>[2x]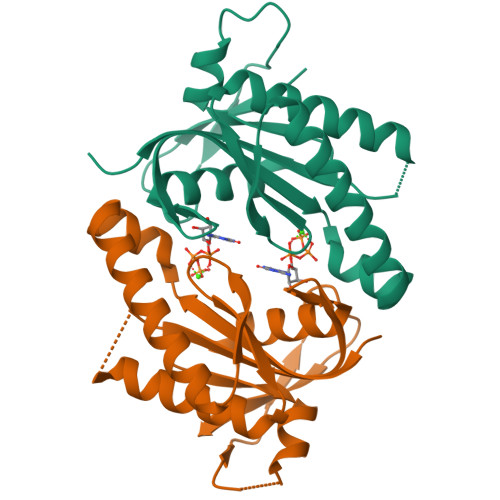FQGAMGSRVVILFTDIEESTALNERIGDRAWVKLISSHDKLVSDLVRRQSGHVVESQGDGFMVAFARPEQAVRCGIELQRALRRNANRKRHEEIRVRIGIHMGRSVRRGDGLFGRNVAMAYRVAAQAAGGEILVSQPVRDALSRSDGIRFDDGREVELKGFSGTYRLFAVLASPDPG>[2x]GPHMGEEAPPGVRSVKVVLVGDGGCGKTSLLMVFADGAFPESYTPTVFERYMVNLQVKGKPVHLHIWDTAGLDDYDRLRPLFYPDASVLLLCFDVTSPNSFDNIFNRWYPEVNHFCKKVPIIVVGCKTDLRKDKSLVNKLRRNGLEPVTYHRGQEMARSVGAVAYLECSARLHDNVHAVFQEAAEVALSSR;>[2x]EYAPLTVSVIVQDEGIDAIPVKVLNCDTISQVKEKIIDQVYRTQPCSCWPKPDSVVLEWRPGSTAQILSDLDLTSQREGRWKRINTLMHYNVRDGATLILSKV

Plexins are semaphorin receptors that play essential roles in mammalian neuronal axon guidance and in many other important mammalian biological processes. Plexin consists of a large multi-domain extracellular module including the ligand-binding Sema domain, a single-pass transmembrane helix, and an intracellular module that includes a GTPase-activating protein (GAP) domain and a Rho-family GTPase-binding domain (RBD). Plexin signaling depends on a semaphorin-induced dimerization mechanism and is modulated by small GTPases of the Rho family, of which RND1 serves as a plexin activator yet its close homolog RhoD an inhibitor. RhoD binds plexin RBD with similar affinity as RND1, but it strongly inhibits plexin signaling rather than activates it.

To experimentally determine the binding mode between plexin and RhoD, a negative plexin regulator, we screened various combinations of RhoD and the intracellular region of plexin family members from different species for crystallization, which resulted in crystals of the complex of mouse plexin B2 and human RhoD bound to the GTP analogue GMP-PNP. Analyses of the diffraction data suggested that plexin B2 degraded during the incubation in crystallization drops, and the crystals only contained the complex between RhoD and the RBD of plexin B2. We solved the structure to 3.1 Å resolution by molecular replacement. The asymmetric unit of the crystal contains two RhoD molecules, each of which binds to one plexin B2 RBD molecule. Surprisingly, the two RBD domains form a domain-swapped dimer in the structure, with the N-terminal portion of one molecule fold together with the C-terminal portion of the other. This domain-swapped dimer is likely a crystallization artifact because it cannot form in the context of a plexin dimer, in which the two RBD domains are far apart from one another. We therefore consider each RBD domain formed by the two halves of the two molecules as a representative of one intact, unswapped RBD as its conformation is very similar to the structures of other RBDs. The structure confirms that RhoD binds the plexin B2 RBD in a mode similar to those of other complexes between Rho-family GTPases and plexin. The GTP analogue GMP-PNP and Mg2+ together stabilize the ligand-binding switch I and switch II regions in the active conformation, which make an extensive interface with one side of the beta-sheet of the RBD. Interestingly, a superimposition of the RhoD/plexin B2-RBD complex with the RND1/plexin B1-RBD complex based on the RBD domains shows that the orientation of RhoD and RND1 relative to the RBD domains is slightly different.>[9x]MTTRLEWAKASPDAYAAMLGLEKALAKAGLERPLIELVYL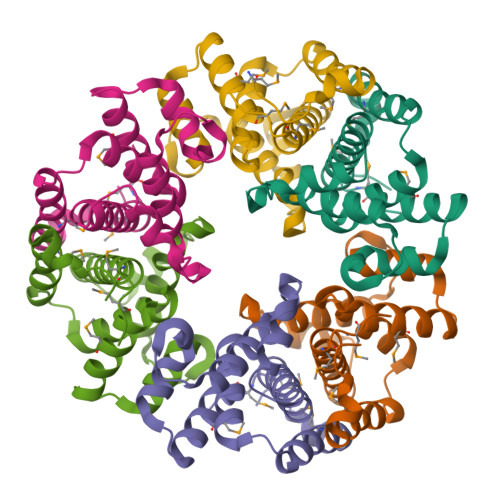RTSQINGCAYCVNMHANDARKAGETEQRLQALCVWQETPYFTPRERAALAWTEQLARLSQGALPHGLLDELREHFDDKEIAELTLAVSAINAWNRFGVGMGMQPE>[2x]MAHHHHHHIPAPRLMWLYRNGDKHDDGTPF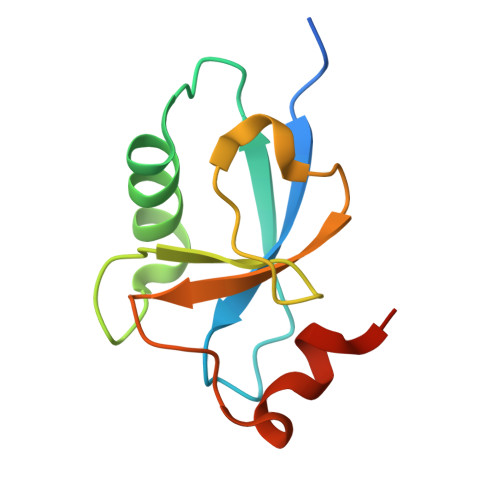FVRPYIKSMESLYQQITKEITPIAGPVRRIFDQNFRVITDLDDIVDGAKYLCTSGEPPAAYDRLEKFLSEWVIQ>SHMGIFSYKDLDENASKALFSDALAISTYAYHNIDNGFDEGYHQTGFGLGLPLTLITALIGSTQSQGGLPGLPWNPDSEQAAQEAVNNAGWSVISATQLGYAGKTDARGTYYGETAGYTTAQAEVLGKYDSEGNLTAIGISFRGTSGPRESLIGDTIGDVINDLLAGFGPKGYADGYTLKAFGNLLGDVAKFAQAHGLSGEDVVVSGHSLGGLAVNSMAAQSDANWGGFYAQSNYVAFASPTQYEAGGKVINIGYENDPVFRALDGTSLTLPSLGVHDAPHTSATNNIVNFNDHYASDAWNLLPFSILNIPTWLSHLPFFYQDGLMRVLNSEFYSLTDKDSTIIVSNLSNVTRGNTWVEDLNRNAETHSGPTFIIGSDGNDLIKGGKGNDYLEGRDGDDIFRDAGGYNLIAGGKGHNIFDTQQALKNTEVAYDGNTLYLRDAKGGITLADDISTLRSKETSWLIFNKEVDHQVTAAGLKSDSGLKAYAAATGGDGDDVLQARSHDAWLFGNAGNDTLIGHAGGNLTFVGGSGDDILKGVGNGNTFLFSGDFGRDQLY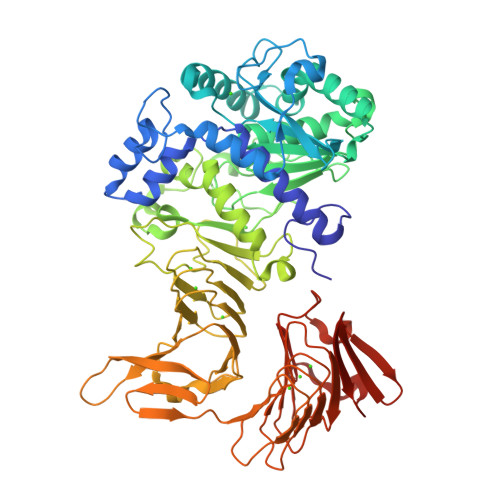GFNASDKLVFIGTEGASGNIRDYATQQNDDLVLAFGHSQVTLIGVSLDHISTDQVVLA[6x]> AEIYNKDGNKVDLYGKAVGLHYFSKGNGENSYGGNGDMTYARLGFKGETQINSDLTGYGQWEYNFQGNNSEGADAQTGNKTRLAFAGLKYADVGSFDYGRNYGVVYDALPEFGGDTAYSDDFFVGRVGGVATYRNSNFFGLVDGLNFAVQYLGKNERDTARRSNGDGVGGSISYEYEGFGIVGAYGAADRTNLQEAQPLGNGKKAEQWATGLKYDANNIYLAANYGETRNATPITNKFTNTSGFANKTQDVLLVAQYQFDFGLRPSIAYTKSKAKDVEGIGDVDLVNYFEVGATYYFNKNM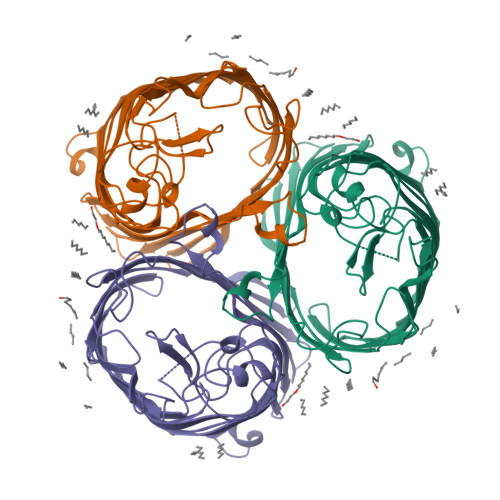STYVDYIINQIDSDNKLGVGSDDTVAVGIVYQF>[2x]AAPPAPPVSYGVEEDVFHPVRAKQGMVASVDATATQVGVDILKEGGNAVDAAVAVGYALAVTHPQAGNLGGGGFMLIRSKNGNTTAIDFREMAPAKATRDMFLDDQGNPDSKKSLTSHLASGTPGTVAGFSLALDKYGTMPLNKVVQPAFKLARDGFIVNDALADDLKTYGSEVLPNHENSKAIFWKEGEPLKKGDTLVQANLAKSLEMIAENGPDEFYKGTIAEQIAQEMQKNGGLITKEDLAAYKAVERTPISGDYRGYQVYSMPPPSSGGIHIVQILNILENFDMKKYGFGSADAMQIMAEAEKYAYADRSEYLGDPDFVKVPWQALTN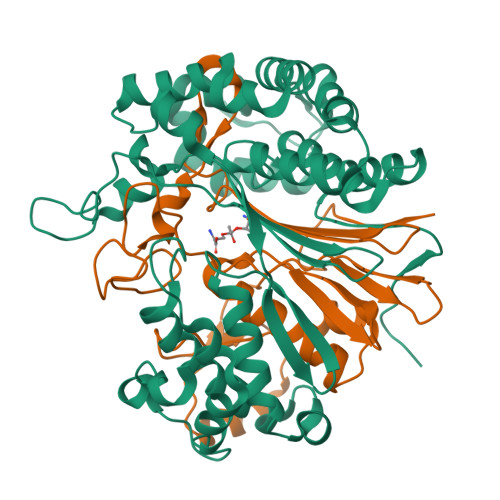KAYAKSIADQIDINKAKPSSEIRPGKLAPYESNQ;>TTHYSVVDKDGNAVAVTYTLNTTFGTGIVAGESGILLNNQMDDFSAKPGVPNVYGLVGGDANAVGPNKRPLSSMSPTIVVKDGKTWLVTGSPGGSRIITTVLQMVVNSIDYGLNVAEATNAPRFHHQWLPDELRVEKGFSPDTLKLLEAKGQKVALKEAMGSTQSIMVGPDGELYGASDPRSVDDLTAGY[2x]> DPDTAVTNKQSFSTDVIYQVFTD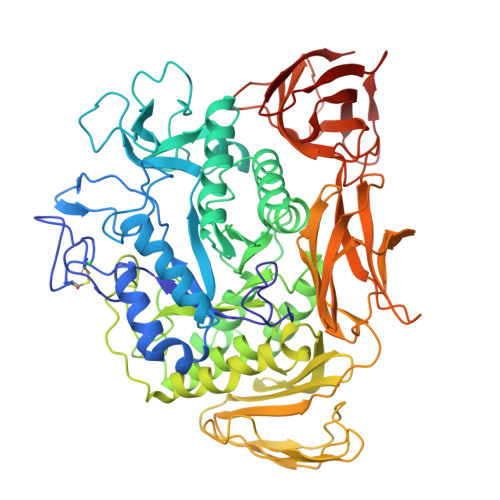RFLDGNPSNNPTGAAYDATCSNLKLYCGGDWQGLINKINDNYFSDLGVTALWISQPVENIFATINYSGVTNTAYHGYWARDFKKTNPYFGTMADFQNLITTAHAKGIKIVIDFAPNHTSPAMETDTSFAENGRLYDNGTLVGGYTNDTNGYFHHNGGSDFSSLENGIYKNLYDLADFNHNNATIDKYFKDAIKLWLDMGVDGIRVDAVKHMPLGWQKSWMSSIYAHKPVFTFGEWFLGSAASDADNTDFANKSGMSLLDFRFNSAVRNVFRDNTSNMYALDSMINSTATDYNQVNDQVTFIDNHDMDRFKTSAVNNRRLEQALAFTLTSRGVPAIYYGTEQYLTGNGDPDNRAKMPSFSKSTTAFNVISKLAPLRKSNPAIAYGSTQQRWINNDVYVYERKFGKSVAVVAVNRNLSTSASITGLSTSLPTGSYTDVLGGVLNGNNITSTNGSINNFTLAAGATAVWQYTTAETTPTIGHVGPVMGKPGNVVTIDGRGFGSTKGTVYFGTTAVTGAAITSWEDTQIKVTIPSVAAGNYAVKVAASGVNSNAYNNFTILTGDQVTVRFVVNNASTTLGQNLYLTGNVAELGNWSTGSTAIGPAFNQVIHQYPTWYYDVSVPAGKQLEFKFFKKNGSTITWESGSNHTFTTPASGTATVTVNWQ2-amino-8-{[2-(4-methoxyphenyl)-2-oxoethyl]sulfanyl}-1,9-dihydro-6H-purin-6-one 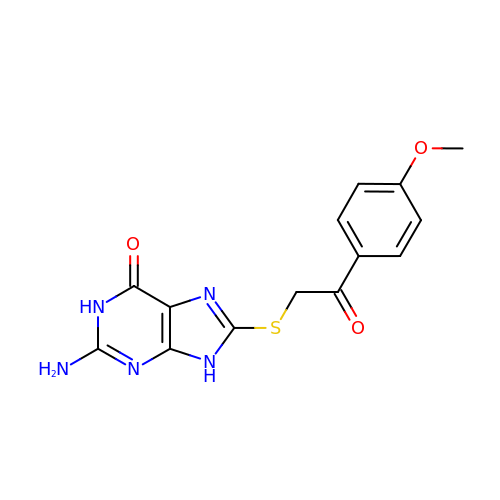| C14 H13 N5 O3 S | SQNJCPSJSYBCFC-UHFFFAOYSA-N> GAMEKFKTLLYDIPIECMEVSEEIISYAKLQLGKKLNDSIYVSLTDHINFAIQRNQKGLDIKNALLWETKRLYKDEFAIGKEALVMVKNKTGVSLPEDEAGFIALHIVNAELNEEMPNIINITKVMQEILSIVKYHFKIEFNEESLHYYRFVTHLKFFAQRLFNGTHMESQDDFLLDTVKEKYHRAYECTKKIQTYIEREYEHKLTSDELLYLTIHIE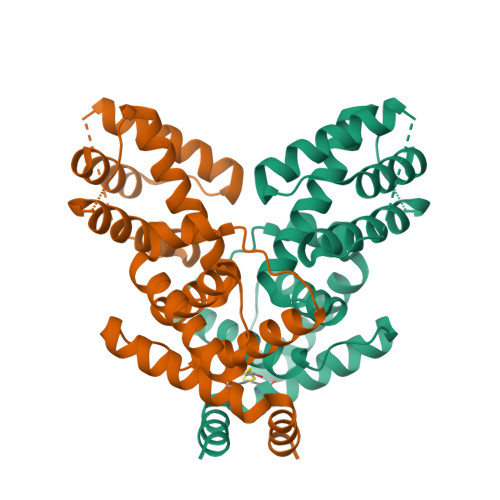RVV> GSFVEMVDNLRGKSGQGYYVEMTVGSPPQTLNILVDTGSSNFAVGAAPHPFLHRYYQRQLSSTYRDLRKGVYVPYTQGKWEGELGTDLVSIPHGPNVTVRANIAAITESDKFFINGSNWEGILGLAYAEIARPDDSLEPFFDSLVKQTHV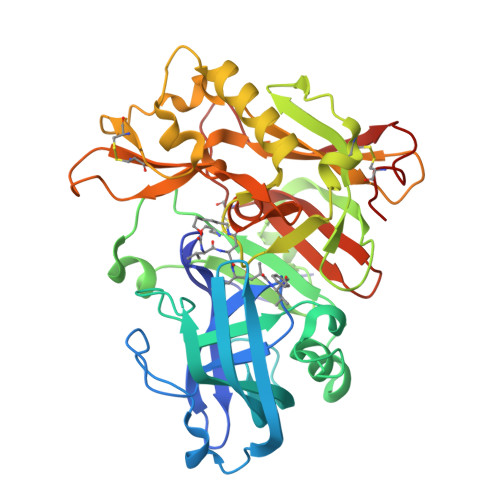PNLFSLQLCGAGFPLNQSEVLASVGGSMIIGGIDHSLYTGSLWYTPIRREWYYEVIIVRVEINGQDLKMDCKEYNYDKSIVDSGTTNLRLPKKVFEAAVKSIKAASSTEKFPDGFWLGEQLVCWQAGTTPWNIFPVISLYLMGEVTNQSFRITILPQQYLRPVEDVATSQDDCYKFAISQSSTGTVMGAVIMEGFYVVFDRARKRIGFAVSACHVHDEFRTAAVEGPFVTLDMEDCGYN>MYTNSDFVVIKALEDGVNVIGLTRGADTRFHHHEHLDKGEVLIAQFTEHTSAIKVRGKAYIQTRHGVIESEGKK[264x]

TRAP has proved a useful building block for construction of artificial nanostructures. The wild‐type protein forms a ring‐shaped assembly comprising 11 identical monomers. We have shown that cysteine‐modified variants of the trp RNA binding attenuation protein, assemble into cage‐like structures with Au(I) or Hg(II), called TRAP‐cage, disassembly of which can be induced by thiol‐ or phosphine‐containing compounds. Here, we report variants of TRAP which can assemble into TRAP‐cages mediated by Co(II) or Zn(II).

Based on the crystal structure of wild‐type TRAP, a histidine residue was introduced at position 33 of the TRAPK35C variant, yielding TRAPS33H/K35C, where the histidine and cysteine residues are located at i and i+2 positions of the β‐sheet motif around the rim of the ring‐shaped structure. The cysteine residue at position 35 of TRAPS33H/K35C was further changed to histidine, resulting in another variant, TRAPS33H/K35H, possessing a pair of imidazole ligands. When the TRAPS33H/K35H protein was mixed with Co(II) or Zn(II), it showed the formation of pseudospherical cages with a diameter of ≈22 nm, similar to TRAP Au(I) 24‐cage. We constructured a number of cages named as follows: Cages made with Zn(II) (TRAPK35C‐Zn(II)‐cages); TRAPS33H/K35H with either Co(II) or Zn(II) (TRAPS33H/K35H‐Co(II) or ‐Zn(II)‐cages); TRAPS33H/K35C with Zn(II) (TRAPS33H/K35C‐Zn(II)‐cages). To verify our designs, we solved the structures of TRAPS33H/K35H‐Zn(II)‐cage, TRAPS33H/K35H‐Co(II)‐cage, and TRAPK35C‐Zn(II)‐cages using cryoEM single particle reconstruction (see Methods for sample preparation and Figures S2–S4 for analysis pipelines). The resulting structures showed that these cages are mainly composed of 24 TRAP rings, and the overall shape and bonding network between adjacent rings is retained when compared to the TRAPAu(I) 24‐cage. They form two chiral cages, and each ring forms two metal‐mediated bridges with each neighbor. In the structure of TRAPS33H/K35H‐Co(II)‐cage, every bridge has in its center one ion in close proximity to the histidine residues introduced in positions 33 and 35 as expected. However, a closer analysis revealed that the coordination geometry is unlikely to be a perfect tetrahedron but rather a distorted one or an octahedron formed by 4 histidine ligands from the protein and 2 bonds with other ligands such as water molecules (which are not visible due to limited resolution). TRAP‐cages that possess only histidine ligands, TRAPS33H/K35H‐Co(II) cages, and TRAPS33H/K35H‐Zn(II) cages, almost completely disassembled in the presence of 35 µM EDTA (1 equivalent to TRAP monomer). TRAPS33H/K35H‐Co(II) and Zn(II)‐cages were more sensitive to pH, disassembling completely at pHs below 4–6 and above 8–10.>[2x]HVSVKPAESAAGSWETYTMKVPSEKNLPTTKVVLKMPKDVEFQQYEPIPG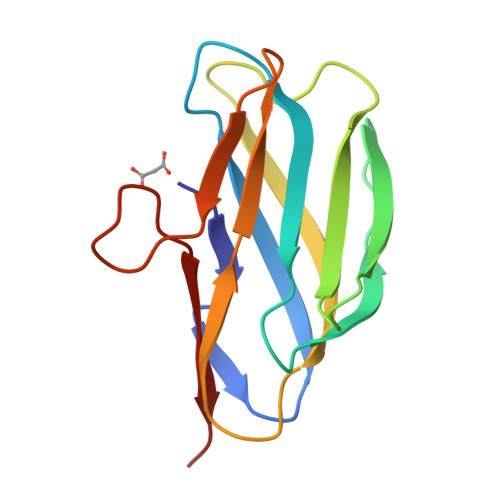WKVSTQKHDDKSVSVTWEATDGGIQEGQFQQFTFVAKNPDKAEEAAWDAYQYYKDGSIVEWTGDEDADTPHSITNITSA> MKQYLELMQKVLDEGTQKNDRTGTGTLSIFGHQMRFNLQDGFPLVTTKRCHLRSIIHELLWFLQGDTNIAYLHENNVTIWDEWADENGDLGPVYGKQWRAWPTPDGRHIDQITTVLNQLKNDPDSRRIIVSAWNVGELDKMALAPCHAFFQFYVADGKLSCQLYQQSCDVFLGLPFNIASYALLVHMMAQQCDLEVGDFVWTGGDTHLYSNH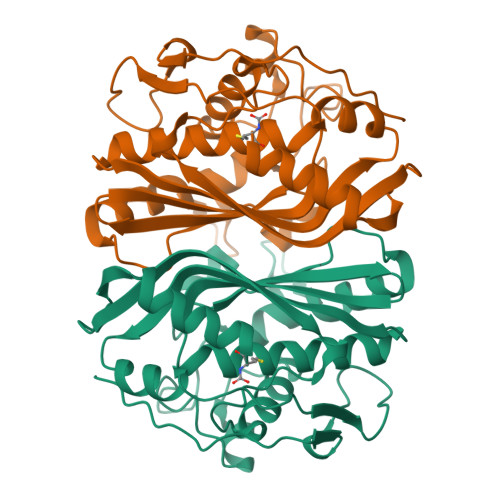MDQTHLQLSREPRPLPKLIIKRKPESIFDYRFEDFEIEGYDPHPGIKAPVAI>MSFSQAVSGLNAAATNLDVIGNNIANSATYGFKSGTASFADMFAGSKVGLGVKVAGITQDFTDGTTTNTGRGLDVAISQNGFFRLVDSNGSVFYSRNGQFKLDENRNLVNMQGMQLTGYPATGTPPTIQQGANPAPITIPNTLMAAKSTTTASMQINLNSTDPVPSKTPFSVSDADSYNKKGTVTVYDSQGNAHDMNVYFVKTKDNEWAVYTHDSSDPAATAPTTASTTLKFNENGILESGGTVNITTGTINGATAATFSLSFLNSMQQNTGANNIVATNQNGYKPGDLVSYQINNDGTVVGNYSNEQEQVLGQIVLANFANNEGLASQGDNVWAATQASGVALLGTAGSGNFGKLTNGALEASNVDLSKELVNMIVAQRNYQSNAQTIKTQDQILNTLVNLR[22x]

The axial structure consists of three morphologically distinct regions, the rod, the hook, and the filament from the proximal to the distal end, with a few minor components. The function of the hook is a universal joint that transmits motor torque to the filament in any orientation relative to the motor axis. The rod is a drive shaft that penetrates the peptidoglycan (PG) layer and the outer membrane and connects the hook with the rotor of the motor. The distal rod and hook show distinct mechanical properties, although they share the same helical symmetry and repeat distance and are composed of similar subunit proteins (FlgG and FlgE) with 39% sequence identity.

The previous cryoEM map of the St-hook also showed an unassigned elongated density between the D1 domain and the D0 helices. The shape and position of the density is very similar to the density corresponding to the l-stretch of the Cj-hook or that of the St-rod. The D0 helices and the l-stretch of Cj-FlgE were well fitted into the EM density with slight modification. The amino acid sequence alignment indicates that the l-stretch of St-FlgE is 18 residues shorter than that of Cj-FlgE. Consistent with this, the density of St-FlgE corresponding to the l-stretch is shorter than the other two and terminates at the position expected from the sequence. Thus, we built the model of the Dc region based on the Cj-FlgE structure and constructed a full-length St-hook model. The subunit interaction mediated by the l-stretch is not as extensive as in the distal rod. The l-stretch extends to the −5 direction and interacts with the inner surface of the D1 domains of the FlgE subunits in the −5 and −11 positions but not with the subunits in −10 and −16 positions. In contrast, the l-stretch of FlgE is shorter than that of FlgG and only interacts with the inner surface of the −5 and −10 subunits. These interactions probably reinforce the hook structure while allowing the axial compression and extension of each hook protofilament for the bending flexibility of the hook.> QDADKLPHTKVTLVAPPQVHPHEQATKSGPKVVEFTMTIEEKKMVIDDKGTTLQAMTFNGSMPGPTLVVHEGDYVQLTLVNPATNAMPHNVNFHGATGALGGAKLTNVNPGEQATLRFKADRSGTFVYHCAPEGMVPWHVVSGMSGTLMVLPRDGLKDPQGKPLHYDRAYTIGEFDLYIPKGPDGKYKDYATLAESYGDTVQVMRTLTPSHIVFNGKVGALTGANALTAKVGETVLLI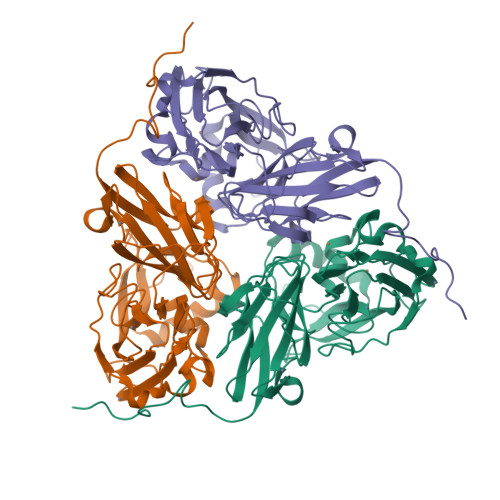HSQANRDTRPHLIGGHGDWVWETGKFANPPQRDLETWFIRGGSAGAALYTFKQPGVYAYLNHNLIEAFELGAAGHIKVEGKWNDDLMKQIKAPAPIPR> GSHMSFLTVPYKLPVSLSVGSCVIIKGTLIDSSINEPQ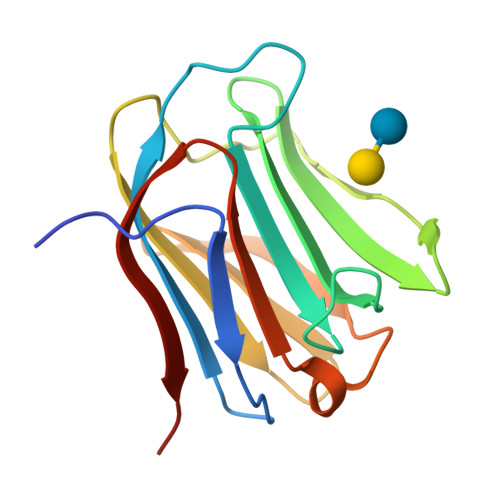LQVDFYTEMNEDSEIAFHLNVRLGRRVVMNSREFGIWMLEENLHYVPFEDGKPFDLRIYVCLNEYEVKVNGEYIYAFVHRIPPSYVKMIQVWRDVSLDSVLVNNGRR>[2x]ASEIELVFRPHPTLME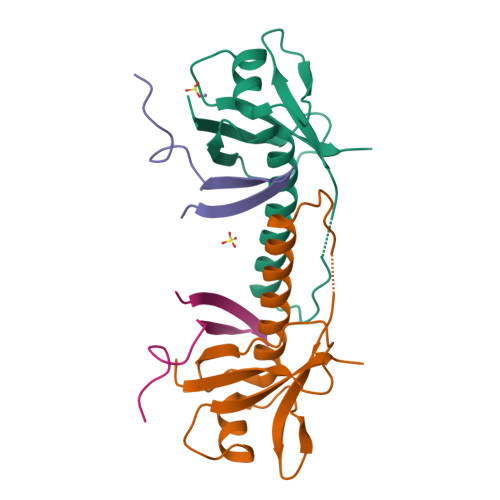KDDSAQTRYIKTSGNATVDHLSKYLAVRLALEELRSKGESNQMNLDTASEKQYTIYIATASGQFTVLDGSFSLELVSEKYWKVNKPMELYYAPTK;>EVTVTDITANSITVTFREAQAAEGFFRDRS[2x]>[2x]SNAMQNKRDSYNREDLLASSQGELFGEGYPQLPAPNMLMMDRITKMSETEGEFGKGLIL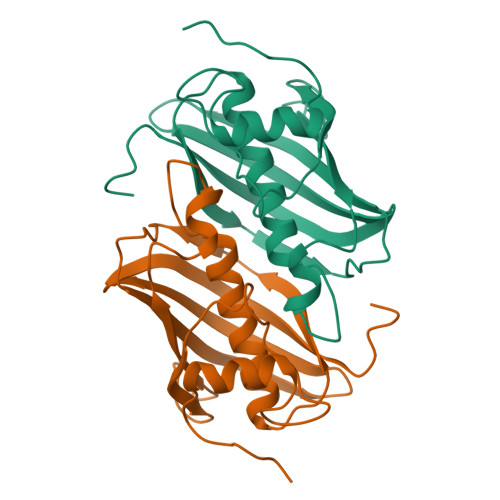AELDITPDLWFFDCHFPGDPVMPGCLGLDAMWQLVGFFLGWVGGKGKGRALGVGEVKFTGQILPTAKKVTYEINMKRVVNRKLVMGLADGRVLVDGKEIYVAKDLKVGLFQDTSAF>SFKDLNLTDAQKQQIREIMKGQRDQMKRPPLEERRAMHDIIASDTFDKVKAEAQIAKMEEQRKANMLALMETQNKIYNILTPEQKKQFNANFEKRLT[2x]

Spy is one of a group of chaperones that allow clients to fold while remaining continuously bound to the surface of the chaperone. We have previously observed that the chaperone substrate Im7 exists in a heterogeneous, largely disordered crystallographic ensemble while bound to the chaperone Spy. To refine strategies for detecting anomalous scattering for observing partially occupied disordered states, we co-crystallized the tight-binding Spy H96L variant with short peptides derived from its client, Im7. These peptides each had a single iodophenylalanine substitution at position 18, 19 or 20.

The Im7 peptides L18pI-Phe and K20pI-Phe crystallized in complex with Spy show a very different pattern compared with the multiple signals observed for L19pI-Phe. The 5.2 keV phased anomalous difference Fourier maps of L18pI-Phe and L20pI-Phe each show only one distinct anomalous signal attributable to iodine. In both cases the peak heights in the phased anomalous difference Fourier maps were very strong: the iodine signals were detected at 26.4σ and 32.5σ for L18pI-Phe and K20pI-Phe, respectively. For K20pI-Phe, a second data set was collected below the iodine edge at 4.5 keV. To further validate this observation, we collected a third data set at an additional goniometer κ angle (κ = −20°) above the iodine edge. Consistent with the L19pI-Phe data collections, the strength of the iodine anomalous signal detected is highly dependent on the crystal quality. This combination of measurements confirmed that K20pI-Phe produced detectable anomalous scattering from a single position in the crystal, providing an ideal case for determining the position of a partially occupied anomalous scatterer. The larger peak heights for L18pI-Phe and K20pI-Phe, compared with each of the L19pI-Phe peaks, suggest a higher level of occupancy at these positions. Anomalous site refinements show that the occupancies of L18pI-Phe and K20pI-Phe are approximately 20% and 33%, with B factors of approximately 47 and 55 Å2, respectively. In the case of K20pI-Phe, a simultaneous fitting of the new L19pI-Phe and K20pI-Phe signals within 0.43 Å on average was possible. However, cross-validation tests in which the K20pI-Phe signal was held out did not back-predict the K20pI-Phe anomalous signal.>[2x]HHHHHHMSAIENFDAHTPMMQQYLRLKAQHPEILLFYRMGDFYELFYDDAKRASQLLDISLTKRGASAGEPIPMAGIPYHAVENYLAKLVNQGESVAICEQIGDPATSKGPVERKVVRIVTPGTISDEALLQERQDNLLAAIWQDSKGFGYATLDISSGRFRLSEPADRETMAAELQRTNPAELLYAEDFAEMSLIEGRRGLRRRPLWEFEIDTARQQLNLQFGTRDLVGFGVENAPRGLCAAGCLLQY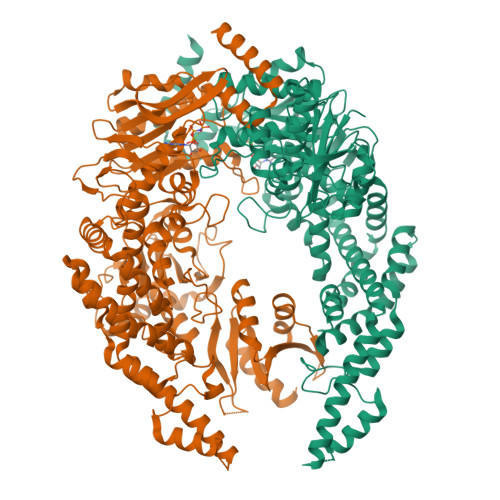AKDTQRTTLPHIRSITMEREQDSIIMDAATRRNLEITQNLAGGAENTLASVLDCTVTPMGSRMLKRWLHMPVRDTRVLLERQQTIGALQDFTAGLQPVLRQVGDLERILARLALRTARPRDLARMRHAFQQLPELRAQLETVDSAPVQALREKMGEFAELRDLLERAIIDTPPVLVRDGGVIASGYNEELDEWRALADGATDYLERLEVRERERTGLDTLKVGFNAVHGYYIQISRGQSHLAPINYMRRQTLKNAERYIIPELKEYEDKVLTSKGKALALEKQLYEELFDLLLPHLEALQQSASALAELDVLVNLAERAYTLNYTCPTFIDKPGIRITEGRHPVVEQVLNEPFIANPLNLSPQRRMLIITGPNMGGKSTYMRQTALIALMAYIGSYVPAQKVEIGPIDRIFTRVGAADDLASGRSTFMVEMTETANILHNATEYSLVLMDEIGRGTSTYDGLSLAWACAENLANKIKALTLFATHYFELTQLPEKMEGVANVHLDALEHGDTIAFMHSVQDGAASKSYGLAVAALAGVPKEVIKRARQKLRELESIS3-(3-{2-[(5-METHANESULFONYL-THIOPHENE-2-CARBONYL)-AMINO]-ETHYLDISULFANYLMETHYL}- BENZENESULFONYLAMINO)-4-OXO-PENTANOIC ACID | C20 H24 N2 O8 S5 | 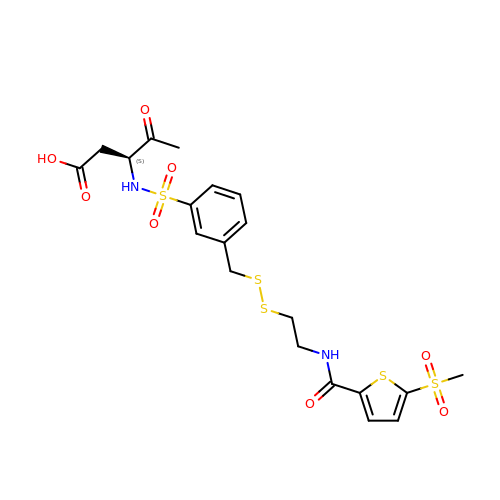VIJJMTFSKSTKFB-INIZCTEOSA-N>[2x]MKFSVIVPTYNSEKYITELLNS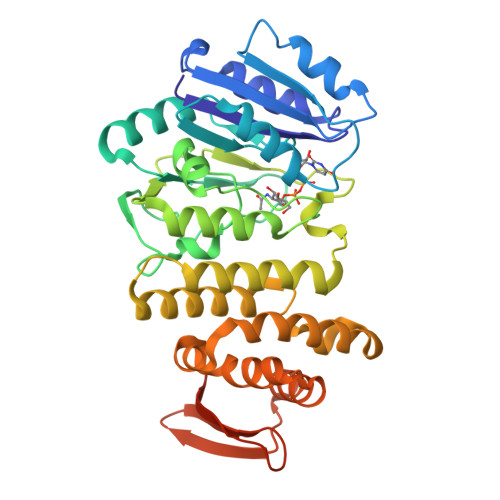LAKQDFPKTEFEVVVVDDCSTDQTLQIVEKYRNKLNLKVSQLETNSGGPGKPRNVALKQAEGEFVLFVDSDDYINKETLKDAAAFIDEHHSDVLLIKMKGVNGRGVPQSMFKETAPEVTLLNSRIIYTLSPTKIYRTALLKDNDIYFPEELKSAEDQLFTMKAYLNANRISVLSDKAYYYATKREGEHMSSAYVSPEDFYEVMRLIAVEILNADLEEAHKDQILAEFLNRHFSFSRTNGFSLKVKLEEQPQWINALGDFIQAVPERVDALVMSKLRPLLHYARAKDIDNYRTVEESYRQGQYYRFDIVDGKLNIQFNEGEPYFEGIDKLVPRGSAAAALEHHHHHH2-(2-fluorophenyl)ethanamine 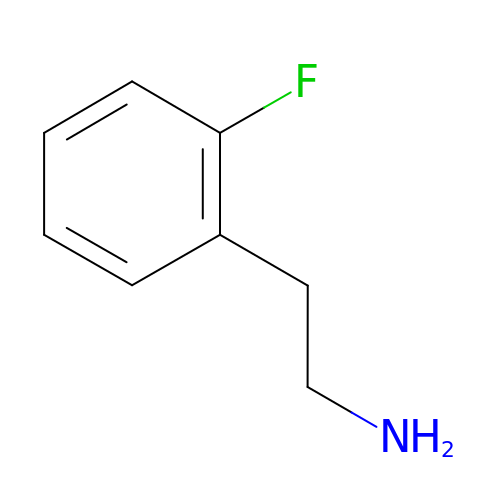| C8 H10 F N | RIKUOLJPJNVTEP-UHFFFAOYSA-N> MATLTDRSYFPPLGECLSGNKIILSWRLVATALEDLACDRLRSAAVSAFLRDGYVHQLLREPTKTFAPPTNETKLDFETKTGAINVVPSPNDPYNLDTIKDDARWLSRNVNINEVAALRVVIIEYQSRAHSHLTGPLSTQDVANVQEAAGVGDAQASAIVALLNVTTVADADSAWADFESETTRRRRLLATYLSERRSFLAAVDALLAFLLHSRAPGTGVELDPLRNAVLQGAFGFDQNAAKPDTTQLDALAPTYIRTLEGCFDRMQMAPESLDNQMLTEQFEVDWIRTALTEAIHAMSLIFQILDLKASQFAAPALVTQWFALMDTCEFFEPVPRGHELIAELLMPLHSLVAAISLKLLNVDRTLSYLDQDVDLLEEEEPYLASSDNLAQMHTTIAAAASAGLISTMPVVFAWSLILHQMHVGYQERAERRDLLQNQRAQAGFELEYEPSGRQRRNSAGSIVSIEASSYDVFLVSQQLERNIEPAENMARIATGRGQVYELMADMAVCLGSGQLAAFRPVLGARARLTFQDLLKRSAHYVGYQAEPVSCLLSILSGGSQYWDISAEAPSNEKSALDIYTRMLSDDTLNVQYASQSRNRFPYEFLPFASMCRILSAALVSDNESSELITGLLVKNPSLTLNWDPRWDRSYELVFEEENTNSFRLTKDIDLFDAASKSNRRILPEEKCTISRGTFGRFVTDVGRVAKLEFEHSTLALFGKRLEVNLMAGAYDTALGYLSADELIEGISLLATVLRAETLRSSKTDPDRGLRILTEASRLLSRGRDIMNVVCDTLDSLVEEELADLDGPKTAALSSCLQFLHAALPVCPGRVWAYMARCPLINTDTRSGRLSRITANLDMLAERYDLLLSAVKLFSSLVDSAKTSAVQRRSGISVNSRAKGEENPWIGASDKIVSRVTLSIAQTSVDVFENSATWRFPSEVDRSVMIRDVVGIMHKLMLYTHSVGSTDTPRSLTGPLAPAADYVVESFLSSSSSSLRFQPLLATLLAAFQLPDTTIYQRRAQIVSERLTTVLEFATILLRVADYLNKASAGIQTQLFKSACVIARLPAIRHSFRIPAISLLSALVESAGKSSGEPPSLLGYLGPQVSRSFIQIAAQLDKPFDRVAEVASTWRFFSTILRNRQQWMANCLLTGKTPREALKGE

Nucleocytoplasmic transport across the nuclear envelope is controlled and facilitated by nuclear pore complexes (NPCs), very large, modular protein assemblies. The Nic96 complex organizes four architectural proteins, Nic96, Nup157/170, Nup188, and Nup192, as well as the more disordered protein Nup53/59. Nup188 is a stacked helical protein with intrinsic flexibility. Moreover, we can show that both Nup188 and Nup192 specifically bind to FG-repeats and translocate across NPCs by facilitated diffusion.

The N-terminal fragment (Nup188N) includes residues 1–1160 and its structure was solved to 2.65 Å resolution. Nup188N crystallized in space group C21 with one copy per asymmetric unit. Nup188N is built from 52 stacked helices. They fold into a large right-handed superhelical ring that resembles a lock washer. We can discern an inner ring of helices forming the concave surface and an outer ring of helices forming the convex surface creating three distinct subdomains. Between helix α32 and α33, we find a β-stranded insertion with structural homology to Src-homology (SH3) domains. The Nup188N ring structure is closed by four helices (α10–α13) from subdomain I that latch onto a complementary surface created by helices α44, α46 and α47. In total, the latch covers an 1511 Å2 interface. In contrast to canonical SH3 domains, the SH3-like domain in Nup188 has a different β-strand topology, which represents a circular permutation. The most regular part of Nup188N is subdomain III, which was found to be structurally similar to nuclear transport receptors (NTRs).>GGILESQFLKEELVVAVEDVRKQGDLMKSAAGEFADDPSSSVKRGNMVRAARALLSAVTRLLILADMADVYKLLVQLKVVEDGILKLRNAGNEQDLGIQYKALKPEVDKLNIMAAKRQQELKDVGNRDQMAAARGILQKNVPILYTASQACLQHPDVAAYKANRDLIYKQLQQAVTGISNAAQATASDDAAQHQGGSGGELAYALNNFDKQIIVDPLSFSEERFRPSLEERLESIISGAALMADSSCTRDDRRERIVAECNAVRQALQDLLSEYMGNAGRKERSDALNSAIDKMTKKTRDLRRQLRKAVMDHVSDSFLETNVPLLVLIEAAKNGNEKEVKEYAQVFREHANKLIEVANLACSISNNEEGVKLVRMSASQLEALCPQVINAALALAAKPQSKLAQENMDLFKEQWEKQVRVLTDAVDDITSIDDFLAVSENHILEDVNKCVIALQEKDVDGLDRTAGAIRGRAARVIHVVTSEMDNYEPGVYTEKVLEATKLLSNTVMPRFTEQVE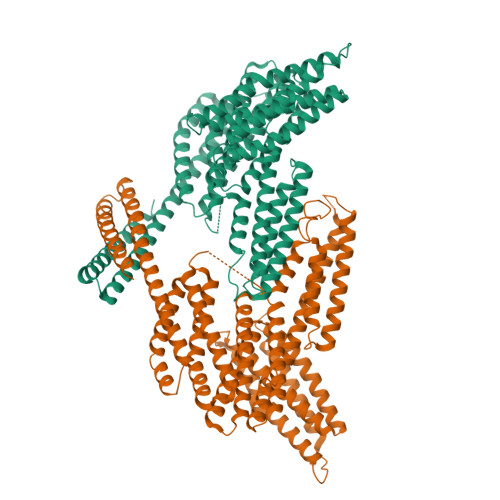AAVEALSSDPAQPMDENEFIDASRLVYDGIRDIRKAVLMIRTPEELDDSDFETEDFDVRSRTSVQTEDDQLIAGQSARAIMAQLPQEQKAKIAEQVASFQEEKSKLDAEVSKWDDSGNDIIVLAKQMCMIMMEMTDFTRGKGPLKNTSDVISAAKKIAEAGSRMDKLGRTIADHCPDSACKQDLLAYLQRIALYCHQLNICSKVKAEVQNLGGELVVSGVDSAMSLIQAAKNLMNAVVQTVKASYVASTKYQKSQGMASLNLPAVSWKMKAPEKKPLVKREKQDETQTKIK[2x]>[4x]MVKEIHVEGFEAYSKAAEENNGKNIFALFCGSKDANGESWC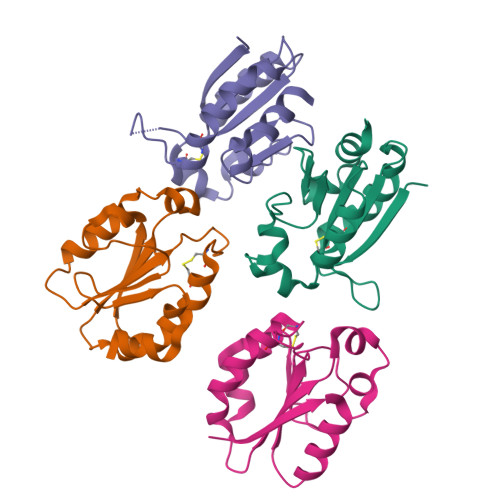PDCVTAEPVIARNLKYAPADSVFIHCSVGERAFWKDQSNVFRKDPVLKLKCVPTLLKPGTPQRLEEEQCADDNLVQMFFQEE> ADRPQIESLSLNGVPNIFLSTKAGGGGSGGGGSGGGGSSAFFFCGAIFECHYLNGTERVRYLQRYI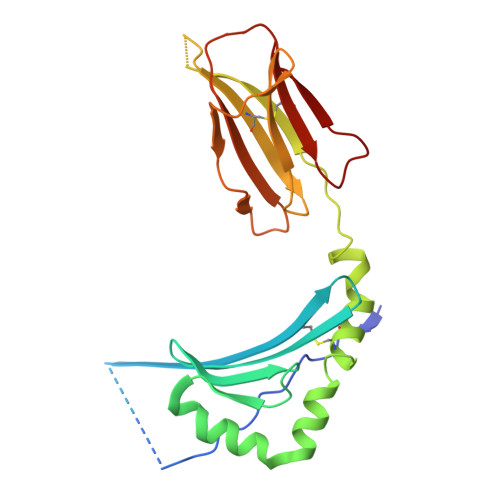YNRQQLVHFDSDVGKFVADTPLGEPQAEYWNSNAELLENIMNIADGSCRHNYGILESFTVQRSVEPKVRVSALQSGSLPETDRLACYVTGFYPPEIEVKWFLNGREETERVVSTDVMQNGDWTYQVLVVLETVPRRGDSYVCRVEHASLRQPISQAWE>GPHMGGSAEVNASPLKHFVTAKKKINGIFEQLGAYIQESATFLEDTYRNAELDPVTTEEQVLDVKGYLSKVRGISEVLARRHMKVAFFGRTSNGKSDVINAMLWDKVLPSGIGHTTNCFLRVEGTDGHEAFLLTEGSEEKRSAKTVNQLAHALHQDKQLHAGSLVSVMWPNSKCPLLKDDLVLMDSPGIDVTTELDSWIDKFCLDADVFVLVANSESTLMQTEKHFFHKVSERLSRPNIFILNNRWDASASEPEYMEEVRRQHMERCTS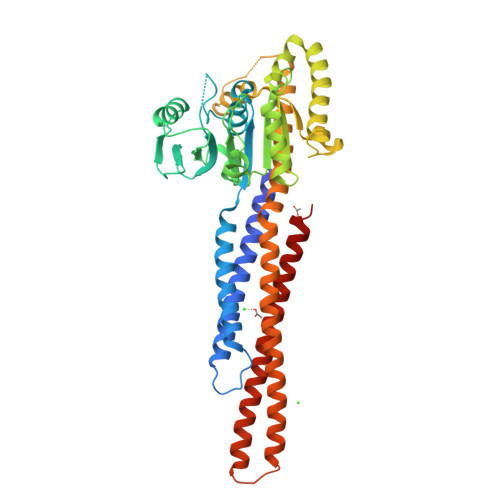FLVDELGVVDRSQAGDRIFFVSAKEVLNARIQKAQGMPEGGGALAEGFQVRMFEFQNFERRFEECISQSAVKTKFEQHTVRAKQIAEAVRLIMDSLHMAAREQQVYCEEMREERQDRTRENLEQEIAAMNKKIEVLDSLQSKAKLLRNKAGWLDSELNMFTHQYLQPSR[2x]>[2x]SNAMDLVQKQKSLQDYTKSLFLEGIL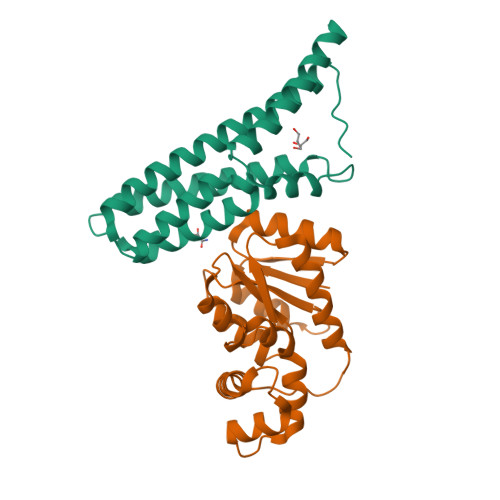DSQFLQLQQLQDESNPDFVSQVVTLFFQDSDRILNDLSLSLDQQVVDFKKVDPHVHQLKGSSSSIGAQRVKNACVVFRSFCEQQNVEACHRCLQQVKQEYYLVKNRLETLFKLEQQIVASGGMIPAVELGF;>MHHHHHHENLYFQSNARVLVVDDDPTCLMILERMLRTCLYEVTKCNRAEMALSLLRKNKHGFDIVISDVHMPDMDGFKLLEHVGLEMDLPVIMMSADDSKSVVLKGVTHGAVDYLIKPVRMEALKNIWQHVVRKRRSEWSVPEHSGSIEETGERQQQQHRGGGGGAAVSGGEDAVDDNSSSVNEGNNWRSSSRKRKDEEGEEQGDDKDEDASNLKKPRVVWSVELHQQFVAAVNQLGVEKAVPKKILELMNVPGLTRENVASHLQKYRIYLRRLG[2x]>[3x]GHMSTPLTLIATITAAPGHAEALERELRALVAPSRAEAGC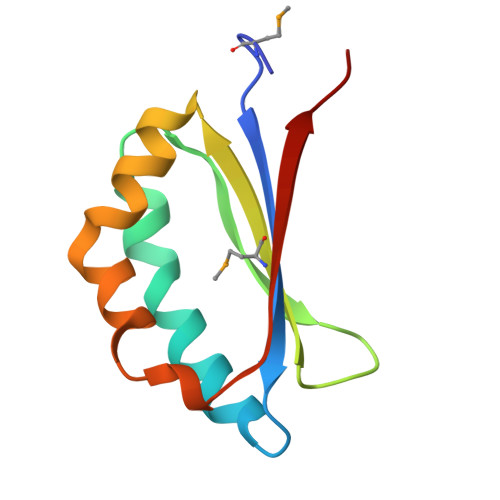LQYDLHQDRHDSHLFYMIEQWRDDAALERHQNTEHFLRFSRGNEALLQNVKIDQLYRLA>GSALVEMYRRAVATGRAAEAVEVLGTVATFRPVFRSPDELGEPPALVPLGTGAGGPTLVCC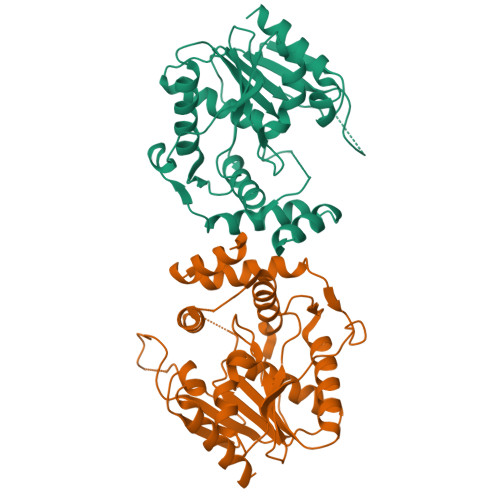AGTAAASGPREFTAFAAALAGLRDVTVLPQTGFLTGEPLPAGLDVLLDAQADAVLAHCAGRPFVLVGHSAGANMAHALTVRLEARGADPAALVLMDIYTPAAPGAMGVWREEMLAWVAERSVVPVDDTRLTAMGAYHRLLLDWAPRPTRAPVLHLYAGEPAGAWPDPRQDWRSRFDGAHTSAEVPGTHFSMMTEHAPVTAATVHKWLDEV[4x]> MFSAGHKIKGTVVLMPKNELEVNPDGSAVDNLNAFLGRSVSLQLISATKADAHGKGKVGKDTFLEGINTSLPTLGAGESAFNIHFEWDGSMGIPGAFYIKNYMQVEFFLKSLTLEAISNQGTIRFVCNSWVYNTKLYKSVRIFFANHTYVPSETPAPLVEYREEELKSLRGNGTGERKEYDRIYDYDVYNDLGNPDKSEKLARPVLGGSSTFPYPRRGRTGRGPTVTDPNTEKQGEVFYVPRDENLGHLKSKDALEIGTKSLSQIVQPAFESAFDLKSTPIEFHSFQDVHDLYEGGIKLPRDVISTIIPLPVIKELYRTDGQHILKFPQPHVVQVSQSAWMTDEEFAREMIAGVNPCVIRGLEEFPPKSNLDPAIYGDQSSKITADSLDLDGYTMDEALGSRRLFMLDYHDIFMPYVRQINQLNSAKTYATRTILFLREDGTLKPVAIELSLPHSAGDLSAAVSQVVLPAKEGVESTIWLLAKAYVIVNDSCYHQLMSHWLNTHAAMEPFVIATHRHLSVLHPIYKLLTPHYRNNMNINALARQSAINANGIIETTFLPSKYSVEMSSAVYKNWVFTDQALPADLIKRGVAIKDPSTPHGVRLLIEDYPYAADGLEIWAAIKTWVQEYVPLYYARDDDVKNDSELQHWWKEAVEKGHGDLKDKPWWPKLQTLEDLVEVCLIIIWIASALHAAVNFGQYPYGGLIMNRPTASRRLLP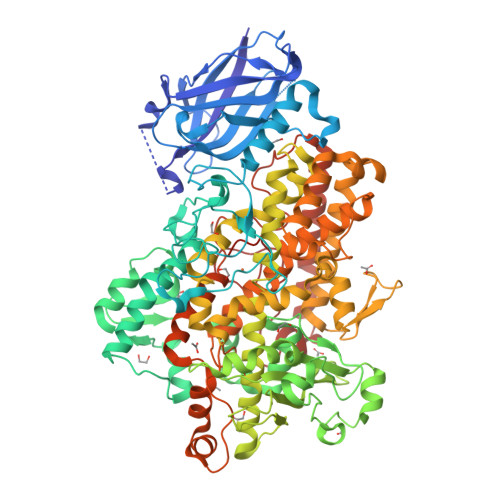EKGTPEYEEMINNHEKAYLRTITSKLPTLISLSVIEIASTHASDEVYLGQRDNPHWTSDSKALQAFQKFGNKLKEIEEKLVRRNNDPSLQGNRLGPVQLPYTLLYPSSEEGLTFRGIPNSISI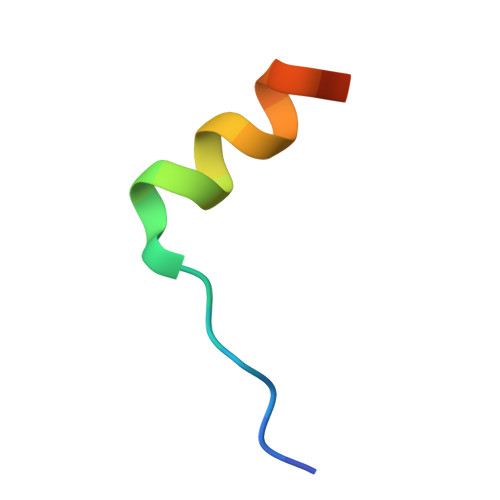> ELPIARRASLHRFLEKRKDRV>EHQKEIQYEILQKTIPTFEPKESILKKLEDIKPEQAKKQTKLFRIFEPRQLPIYRANGEKELRNRWYWKLKKDTLPDGDYDVREYFLNLYDQVLTEMPDYLLLKDMAVENKNSRDAGKVVDSETASICDAIFQDEETEGAVRRFIAEMRQRVQADRNVVNYPSILHPIDYAFNEYFLQHQLVEPLNNDIIFNYIPERIRNDVNYILNMDRNLPSTARYIRPNLLQDRLNLHDNFESLWDTITTSNYILARSVVPDLKELVSTEAQIQKMSQDLQLEALTIQSETQFLTGINSQAANDCFKTLIAAMLSQRTMSLDFVTTNYMSLISGMWLLTVVPNDMFIRESLVACQLAIVNTIIYPAFGMQRMHYRNGDPQTPFQIAEQQIQNFQVANWLHFVNNNQFRQVVIDGVLNQVLNDNIRDGHVINQLMEALMQLSRQQFPTMPVDYKRSIQRGILLLSNRLGQLVDLTRLLAYNYETLMACVTMNMQHVQTLTTEKLQLTSVTSLCMLIGNATVIPSPQTLFHYYNVNVNFHSNYNERINDAVAIITAANRLNLYQKKMKAIVEDFLKRLHIFDVARVPDDQMYRLRDRLRLLPVEVRRLDIFNLILMNMDQIERASDKIAQGVIIAYRDMQLERDEMYGYVNIARNLDGFQQINLEELMRTGDYAQITNMLLNNQPVALVGALPFVTDSSVISLIAKLDATVFAQIVKLRKVDTLKPILYKINSDSNDFYLVANYDWVPTSTTKVYKQVPQQFDFRNSMHMLTSNLTFTVYSDLLAFVSADTVEPINAVAFDNMRIMNEL[2x];>MDVLYSLSKTLKDARDKIVEGTLYSNVSDLIQQFNQMIITMNGNEFQTGGIGNLPIRNWNFDFGLLGTTLLNLDANYVETARNTIDYFVDFVDNVCMDEMVRESQRNGIAPQSDSLIKLSGIKFKRINFDNSSEYIENWNLQNRRQRTGFTFHKPNIFPYSASFTLNRSQPAHDNLMGTMWLNAGSEIQVAGFDYSCAINAPANTQQFEHIVQLRRVLTTATITLLPDAERFSFPRVITSADGATTWYFNPVILRPNNVEIEFLLNGQIINTYQARFGTIIARNFDTIRLSFQLMRPPNMTPAVAALFPNAQPFEHHATVGLTLRIESAVCESVLADASETMLANVTSVRQEYAIPVGPVFPPGM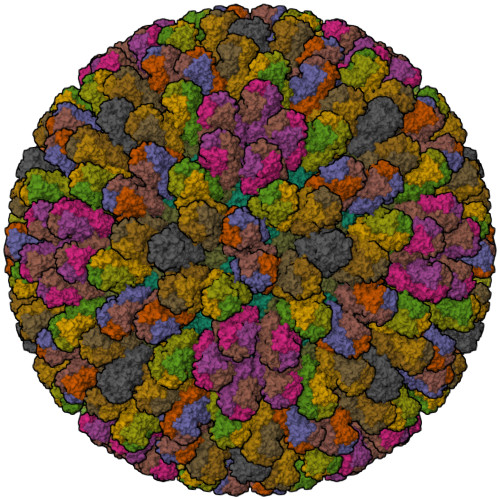NWTDLITNYSPSREDNLQRVFTVASIRSMLVK[13x]> MGDTTQLVKEYQEKRSKLEKFMKNPQHDASLLSNSNEFRDKNVEFFASGGTRTSKFDKLENHPFLGYPYKRG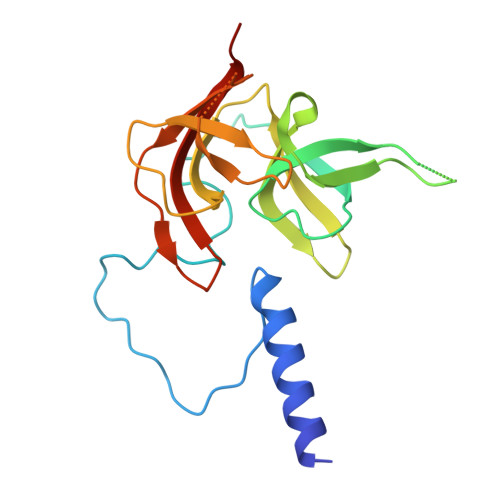VKRVIQEAQDNQSHYEPHVEAGGGEDLYGICIDIDEFSKTATIVPITNNFEGYLVAKDSTVKVKDKLIFNKDGALEKVTGAPNKATINATALTDAKQISNEVYLVKVAVFGNKAMSRN>GG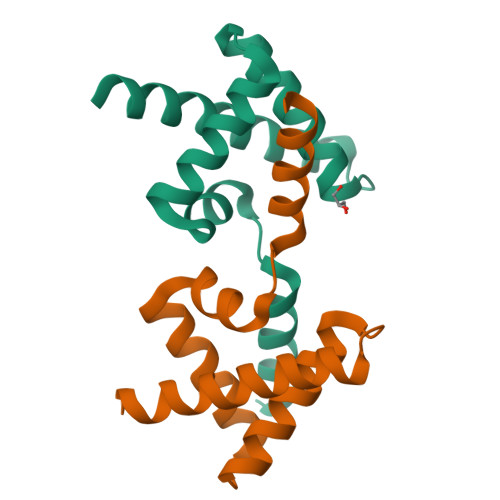HMGEEQKEIETLVELFAEAFREAKRQKKNGTPEEWARDAVEEAARQQGRSRKDVVEALTKYAQEQGRDELLKRLGITPEIYKVIQQIRKEEGSLE[2x]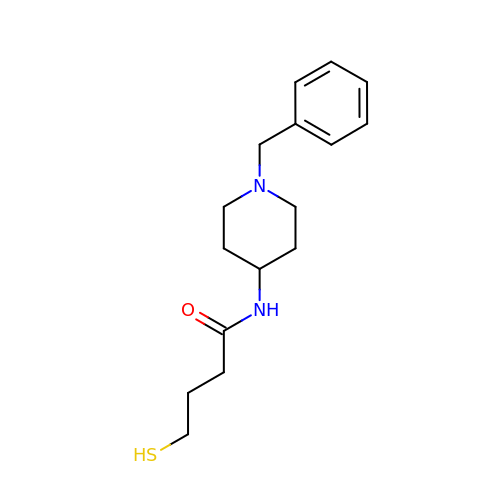N-(1-benzylpiperidin-4-yl)-4-sulfanylbutanamide | C16 H24 N2 O S | XNIXPLIQGKQSIE-UHFFFAOYSA-N>[3x]IHEGILFCIELSETMFKESSDLEYKSPLLEILESLDELMSQLVITRPGTAIGCYFYYCNREDAKEGIYELFPLRDINATFMKKLNDLLEDLSSGRISLYDYFMFQQTGSEKQVRLSVLFTFMLDTFLEEIPGQKQLSNKRVFLFTDIDKPQEAQDIDERARLRRLTIDLFDNKVNFATFFIGYADKPFDNEFYSDILQLGSHTNENTGLDSEFDGPSTKPIDAKYIKSRILRKKEVKRIMFQCPLILDEKTNFIVGVKGYTMYTHEKAGVRYKLVYEHEDIRQEAYSKRKFLNPITGEDVTGKTVKVYPYGDLDINLSDSQDQIVMEAYTQKDAFLKIIGFRSSSKSIHYFNNIDKSSFIVPDEAKYEGSIRTLASLLKILRKKDKIAILWGKLKSNSHPSLYTLSPSSVKDYNEGFYLYRVPFLDEIRKFPSLLSYDDGSEHKLDYDNMKKVTQSIMGYFNLRDGYNPSDFKNPLLQKHYKVLHDYLLQIETTFDENETPNTKKDRMMREDDS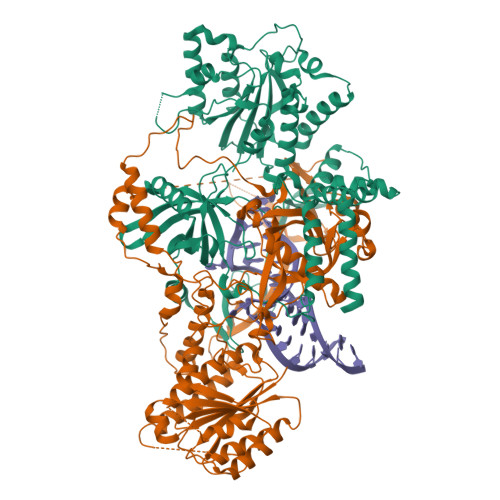LRKLYYIRNKILESEKSEDPIIQRLNKYVKIWNMFYKKFNDDNISIKEEKKPFDKKPKFNI;>[3x]SSESTTFIVDVSPSMMKNNNVSKSMAYLEYTLLNKSKKSRKTDWISCYLANCPVSENSQEIPNVFQIQSFLAPVTTTATIGFIKRLKQYCDQHSHDSSNEGLQSMIQCLLVVSLDIKQQFQARKILKQIVVFTDNLDDLDITDEEIDLLTEELSTRIILIDCGKDTQEERKKSNWLKLVEAIPNSRIYNMNELLVEITSPATSVVKPVRVFSGELRLGADILSTQTSNPSGSMQDENCLCIKVEAFPATKAVSGLNRKTAVEVEDSQKKERYVGVKSIIEYEIHNEGNKKNVSEDDQSGSSYIPVTISKDSVTKAYRYGADYVVLPSVLVDQTVYESFPGLDLRGFLNREALPRYFLTSESSFITADTRLGCQSDLMAFSALVDVMLENRKIAVARYVSKKDSEVNMCALCPVLIEHSNINSEKKFVKSLTLCRLPFAEDERVTDFPKLLDRTTTSGVPLKKETDGHQIDELMEQFVDSMDTDELPEIPLGNYYQPIGEVTTDTTLPLPSLNKDQEENKKDPLRIPTVFVYRQQQVLLEWIHQLMINDSREFEIPELPDSLKNKISPYTHKKFDSTKLVEVLGIKKVDKLKLDSELKTELEREKIPDLETLLKRGEQHSRGSPNNSNN> XWKGYL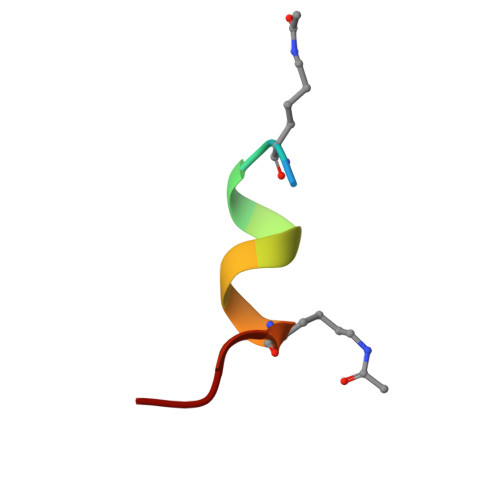CLRKRIQ>[2x]MVSGFAMPKIWRKLAMDIPVNAAKPGRRRYLTLVMIFITVVICYVDRANLAVASAHIQEEFGITKAEMGYVFSAFAWLYTLCQIPGGW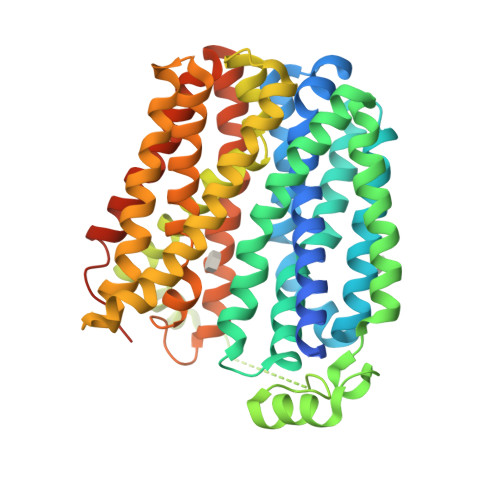FLDRVGSRVTYFIAIFGWSVATLFQGFATGLMSLIGLRAITGIFEAPAFPTNNRMVTSWFPEHERASAVGFYTSGQFVGLAFLTPLLIWIQEMLSWHWVFIVTGGIGIIWSLIWFKVYQPPRLTKGISKAELDYIRDGGGLVDGDAPVKKEARQPLTAKDWKLVFHRKLIGVYLGQFAVASTLWFFLTWFPNYLTQEKGITALKAGFMTTVPFLAAFVGVLLSGWVADLLVRKGFSLGFARKTPIICGLLISTCIMGANYTNDPMMIMCLMALAFFGNGFASITWSLVSSLAPMRLIGLTGGVFNFAGGLGGITVPLVVGYLAQGYGFAPALVYISAVALIGALSYILLVGDVKRVGSLVPRGSGSHHHHHH> MQRRDFLKYSVALGVASALPLWSRAVFAAERPTLPIPDLLTTDARNRIQLTIGAGQSTFGGKTATTWGYNGNLLGPAVKLQRGKAVTVDIYNQLTEETTLHWHGLEVPGEVDGGPQGIIPPGGKRSVTLNVDQPAATCWFHPHQHGKTGRQVAMGLAGLVVIEDDEILKLMLPKQWGIDDVPVIVQDKKFSADGQIDYQLDVMTAAVGWFGDTLLTNGAIYPQHAAPRGWLRLRLLNGCNARSLNFATSDNRPLYVIASDGGLLPEPVKVSELPVLMGERFEVLVEVNDNKPFDLVTLPVSQMGMAIAPFDKPHPVMRIQPIA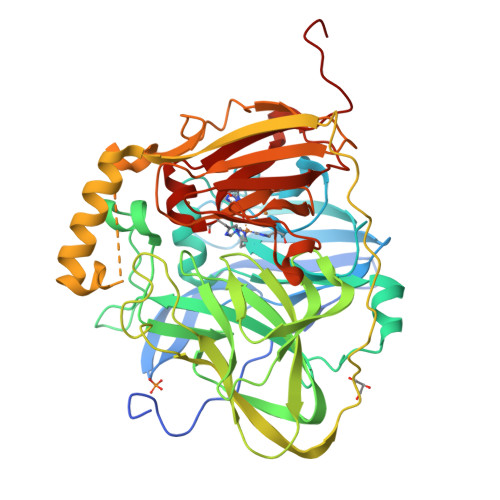ISASGALPDTLSSLPALPSLEGLTVRKLQLSMDPMLDMMGMQMLMEKYGDQAMAGMDHSQMMGHMGHGNMNHMNHGGKFDFHHANKINGQAFDMNKPMFAAAKGQYERWVISGVGDMMLHPFHIHGTQFRILSENGKPPAAHRAGWKDTVKVEGNVSEVLVKFNHDAPKEHAYMAHCHLLEHEDTGMMLGFTVSAWSHPQFEK>SLAKERQKKDNHNLIERRRRFNINDRIKELGTLIPKSNDPDMRWNKGTILKASVDYIRKLQREQQRAKELENRQKKLEHACRHLLLRIQELGIEDFLKVDLRVAKVLSAERVEGSEKLLKLTLSLGDEERTVVAGIAKYYTPEELVGKKIVIVANLKPRKIFGIESQGMILAASDGENLSVIVPDRDVKEGAKLSAALE[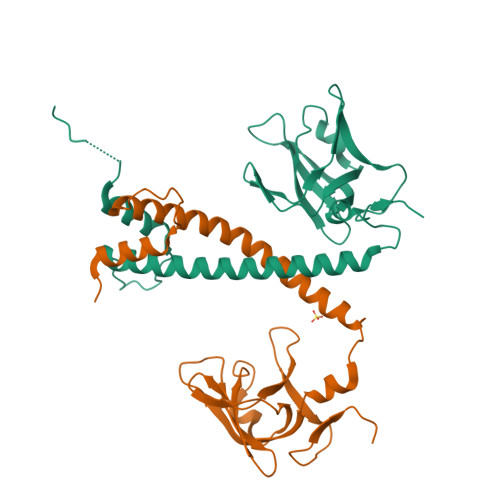4x]>GSHMGTKYKIKETLKRLEDSLRELRRILEELKEMLERLEKNPDKDVIVEVLKVIVKAIEASVENQRISAENQKALAESD[3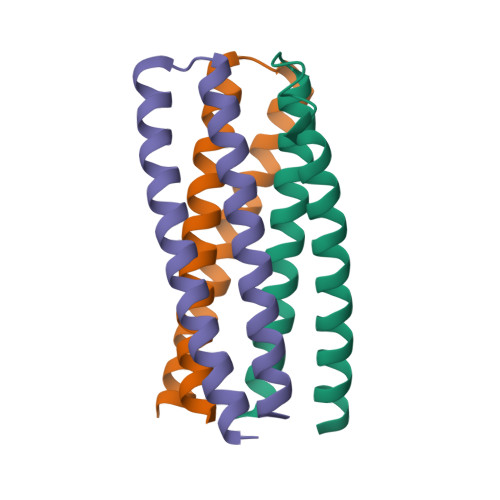x]>QNSHMVKDLNLYAKELVDVVNYLMKKNQLVFSRNNKFIYVNTETIKSMLEKRNYDTVDGKLYLWRELEWIECAE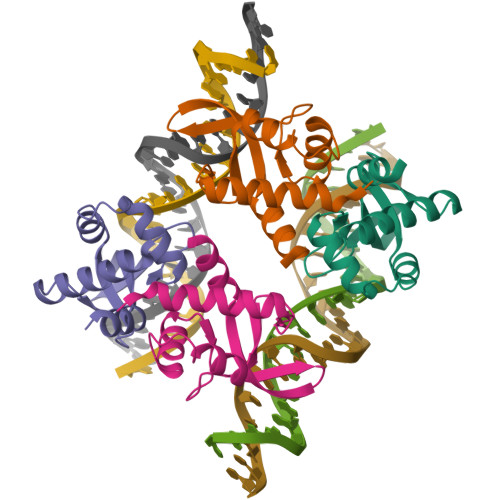DRFNKRIKIDGENMYAVVIKYSSYSILKRLYLE[8x]[(2S,3R,4S,5S,6R)-6-(hydroxymethyl)-2,4,5-tris(oxidanyl)oxan-3-yl]oxy-N-[9-[(2R,3S,5R)-5-[[[(2R,3S)-4-methyl-2,3-bis(oxidanyl)pentanoyl]amino]-oxidanyl-phosphoryl]oxy-3-oxidanyl-oxolan-2-yl]purin-6-yl]phosphonamidic 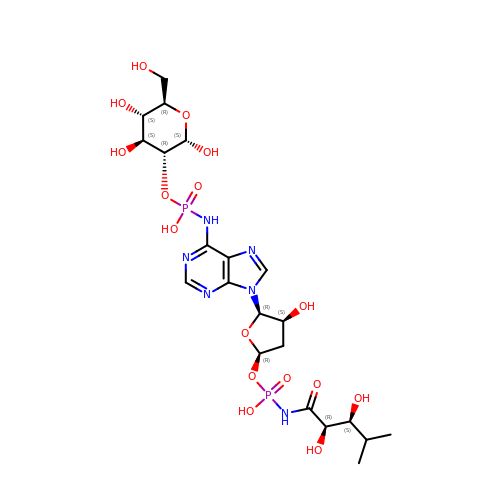acid | C21 H34 N6 O16 P2 | KOMSNTWZRZGGEF-IPMHYPRDSA-N>HLS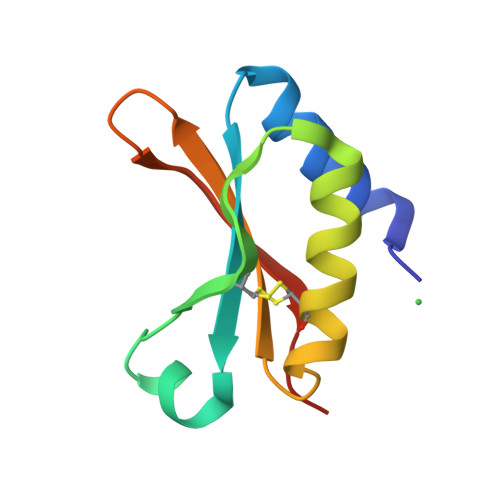LETQEQIRQILSQGHKITFEHVDARRFRTGSWQSCGTLHIDAESDAISTLEACLVDYDGEYVRMVGIDPKGKRRVVETIIQRPNGKN[2x]>SNAMARILKTAYTFDDVLLVPNKSEVLPNEVSLKTQLTKKIQLNIPLMSASMDTVTESKMAIAMAREGGIGIIHKNMTIEDQAREVDRVKRSGGLLCGASIGVTNDMMERVDAVVKAKVDVIVLDTAHGHSKGVIEGVKRIKAKYPELQVIAGNIATPEAVRDLAEAGADCVKVGIGPGSICTTRIVAGVGVPQLTAVMDCAEEGKKLGIPVIADGGLKYSGDIVKALAAGACAAMMGSIFAGCEEAPGAIEIYQGRSYKVYRGMGSLGAMAKGSSDRYFQNGTKKFVPEGVEGRIAYKGHLADTIYQLIGGIKS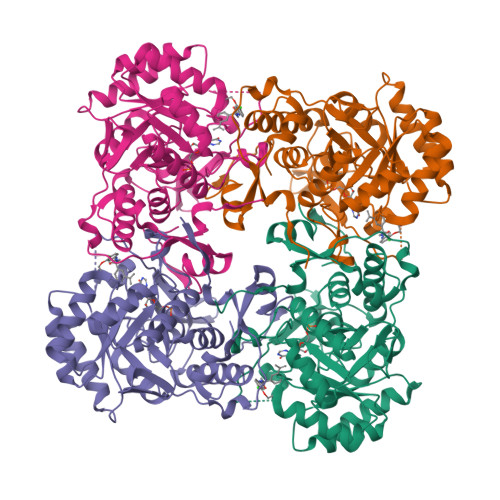GMGYLGAPTLENLYENANFVVQTSAGFRESHPHDINITKEAPNYSVNQ[4x]>[4x]MGSSHHHHHHSQDPNSMGKEILRNPMEAMDPHIFYF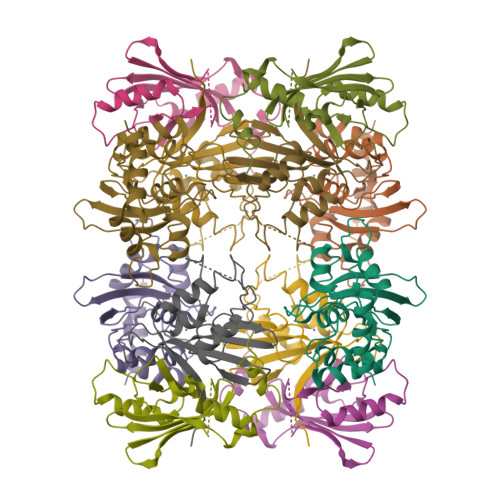HFKNLRKAYGRNESWLCFTMEVVKHHSPVSWKRGVFRNQVDPETGRHAERCFLSWFCDDILSPNTNYEVTWYTSWSPCPECAGEVAEFLARHSNVNLTIKTARLYYFKDTDAAEGLRSLSQEGASVEIMGYKDFKYCWENFVYNDDEPFKPWDGLDYNFLDLDSKLQEILE;>MPRVVPDQRSKFENEEFFRKLSRECEIKYTGFRDRPHEERQARFQNACRDGRSEIAFVATGTNLSLQFFPASWQGEQRQTPSREYVDLEREAGKVYLKAPMILNGVCVIWKGWIDLQRLDGMGCLEFDEERAQQEDALAQQAFEEARRRTR[4x];>MENRWQVMIVWQVDRMRINTWKRLVKHHMYISRKAKDWFYRHHYESTNPKISSEVHIPLGDAKLVITTYWGLHTGERDWHLGQGVSIEWRKKRYSTQVDPDLADQLIHLHYFDEASEGSQIKPPLPSVRKLTEDRWNK[4x]>QDSTSDLIPAPPLSKVPLQQNFQDNQFHGKWYVVGLAGNRILRDDQHPMNMYATIYELKEDKSYNVTSVISSHKKCEYTIATFVPGSQPGEFTLGNIKSYGDKTSYLVRVVSTDYNQYAVVFFKLAEDNAEFFAITIYGRTKELASELKENFIRFSK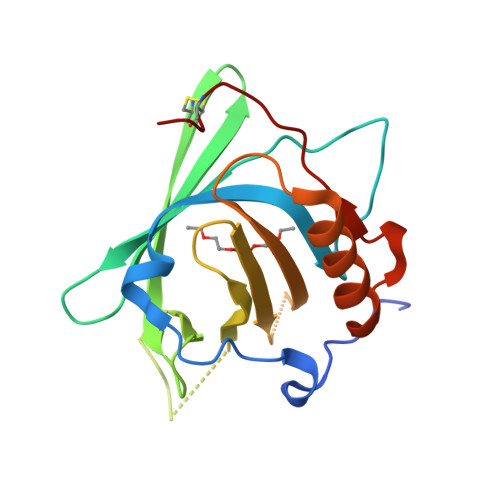SLGLPENHIVFPVPIDQCIDG[8x]> LDFQSESYKDAYSRINAIVIEGEQEAFDNYNRLAEMLPDQRDELHKLAKMEQRHMKGFMACGKNLSVTPDMGFAQKYYERLHENFKAAAAEGKVVTCLLIQSLIIECFAIAAY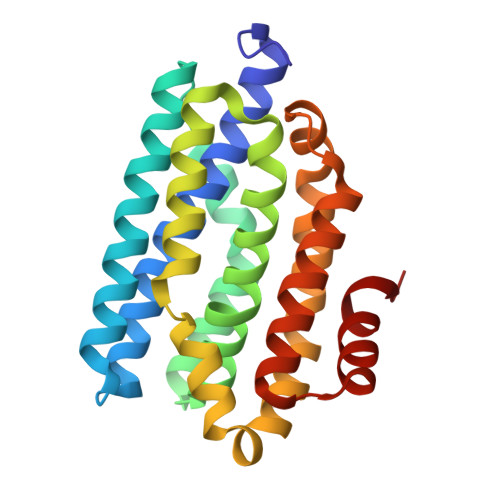NIYIPVADAFARKITEGVVRDEYLHRNFGEEWLKANFDASKAELEEANRQNLPLVWLMLNEVADDARELGMERESLVEDFMIAYGEALENIGFTTREIMRMSAYGLAAV> GTGDGSMLSIPPYYRVKNCNLIVDCQYGSTGKGLLAGYLGALEAPQVLCMAPSPNAGHTLVEEDGTARVHKMLPLGITSPSLERIYLGPGSVIDMDRLLEEYLALPRQVELWVHQNAAVVLQEHRDEEAAGGLAPGSTRSGAGSAFIAKIRRRPGTLLFGEAVRDHPLHGVVRVVDTRTAQDMLFRTRSI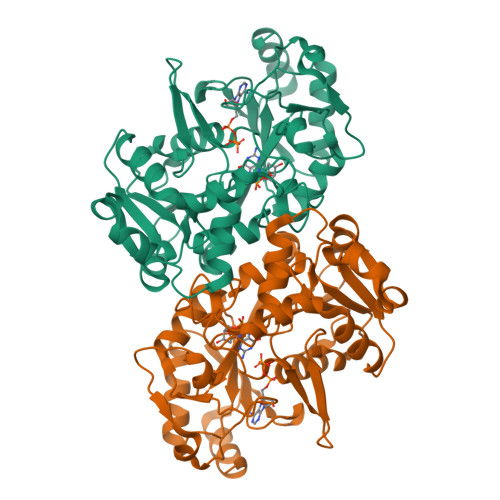QAEGCQGYSLSVHHGAYPYCTARDVTTAQLIADCGLPYDVARIARVVGSMRTYPIRVANRPEAGEWSGPCYPDSVECQFADLGLEQEYTTVTKLPRRIFTFSAIQAHEAIAQNGVDEVFLNFAQYPPSLGALEDILDAIEARAEVTYVGFGPKVTDVYHTPTRAELEGLYARYRR>[5x]MGGWSNFKFLFLSPGGELYGVLNDKIYKGT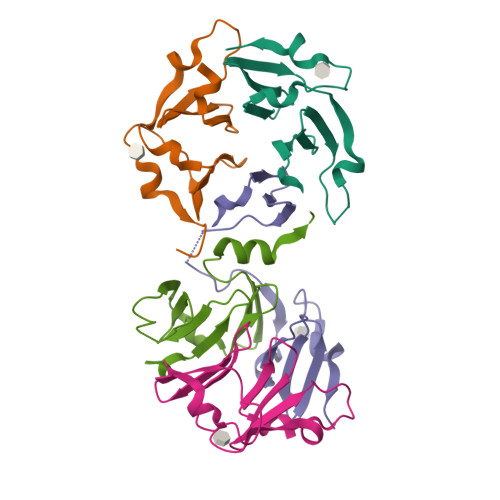PPTHDNDNWLGRAKKIGDGGWNQFQFLFFDPNGYLYAVSKDKLYKAPPPQSDTDNWIARATEIGSGG2-sulfanyl-1,9-dihydro-6H-purin-6-one | C5 H4 N4 O S | 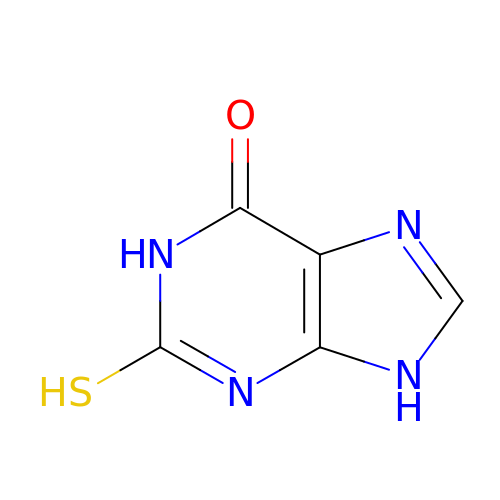XNHFAGRBSMMFKL-UHFFFAOYSA-N>[2x]RAVPGGSSPAWTQCQQLSQKLCTLAWSAHPLVGHMDLREEGDEETTNDVPHIQCGD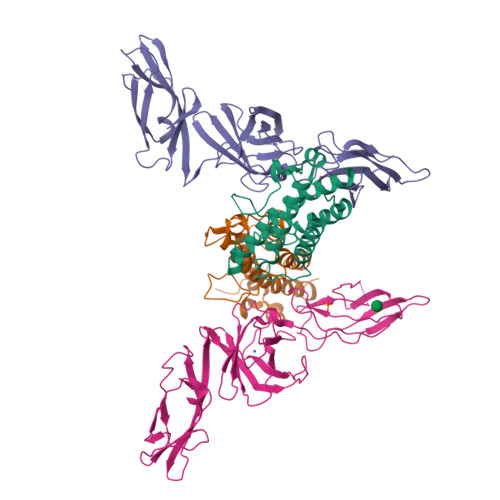GCDPQGLRDNSQFCLQRIHQGLIFYEKLLGSDIFTGEPSLLPDSPVGQLHASLLGLSQLLQPEGHHWETQQIPSLSPSQPWQRLLLRFKILRSLQAFVAVAARVFAHGAATLSPGSHHHHHH;>[2x]IWELKKDVYVVELDWYPDAPGEMVVLTCDTPEEDGITWTLDQSSEVLGSGKTLTIQVKEFGDAGQYTCHKGGEVLSHSLLLLHKKEDGIWSTDILKDQKEPKNKTFLRCEAKNYSGRFTCWWLTTISTDLTFSVKSSRGSSDPQGVTCGAATLSAERVRGDNKEYEYSVECQEDSACPAAEESLPIEVMVDAVHKLKYEQYTSSFFIRDIIKPDPPKNLQLKPLKNSRQVEVSWEYPDTWSTPHSYFSLTFCVQVQGKSKREKKDRVFTDKTSATVICRKNASISVRAQDRYYSSSWSEWASVPCS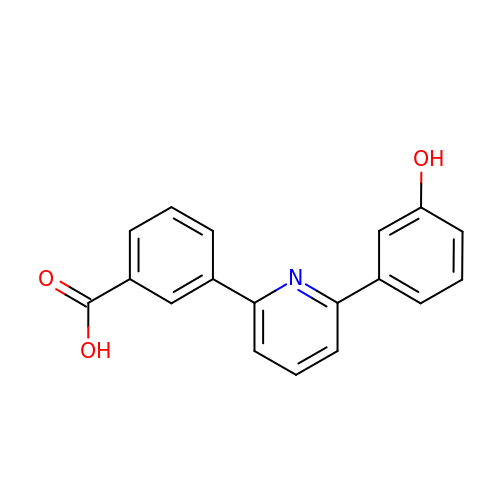3-[6-(3-hydroxyphenyl)pyridin-2-yl]benzoic acid | C18 H13 N O3 | RGVPEEGFSSWQPL-UHFFFAOYSA-N Nucleocytoplasmic transport across the nuclear envelope is controlled and facilitated by nuclear pore complexes (NPCs), very large, modular protein assemblies. The Nic96 complex organizes four architectural proteins, Nic96, Nup157/170, Nup188, and Nup192, as well as the more disordered protein Nup53/59. Nup188 is a stacked helical protein with intrinsic flexibility. Moreover, we can show that both Nup188 and Nup192 specifically bind to FG-repeats and translocate across NPCs by facilitated diffusion.

The C-terminal fragment (Nup188C) includes residues 1445–1827, and we solved its structure to 3.0 Å resolution. Nup188C crystallized in space group P212121 with two copies per asymmetric unit. The C-terminal fragment of Nup188, Nup188C, is a right-handed arc-shaped superhelical structure built from 19 helices that form 6 helical repeats, which are stacked in regular order. The first helical pair (α1 and α2) forms a HEAT repeat followed by 5 ARM repeats. The inner face of the structure is built from helices α2, α5, α8, α12, α15, and α19. The C-terminal helix α19 caps the structure. At the N terminus, helices α1 and α2 expose a hydrophobic surface, which strongly suggests that the full-length protein continues in a stacked pattern. This hydrophobic surface engages in a twofold symmetric crystal packing contact with a neighboring Nup188C molecule resulting in a horseshoe-shaped dimer. Because this contact is generated by a protein truncation, we suggest that it is a crystal artifact and not physiologically relevant. Interestingly, the two Nup188C copies in the asymmetrical unit have a different curvature, likely reflecting the intrinsic flexibility of the molecule.

>SLLPKDISQLLSLVSATINGVDNPWSKDQISYFRTLLKVLFVVLRGTKHSNNAAPQKPTAESPVAVTQLVLTTLDRVVARSFRNLAALVHEPDAATTPEDLALITAILQACLSVPGIEQCQLQVLNIMSSHNVLQVATSLFSWSDRLAEKGDPIYGELALLLLLELSALPALAEQLACDGLLGHLTSANLAGFMRRANVSPFTDNAGAARCYAIWAKGILPLLLNILGALGATIAPEVAFVLNQFPNLLRSSVDRLEAPGLSRTVPLSSRDAPGAGPHYFVALVALSEVHSLALLTRVLAALRSGNARDIPEVVWDSGAVLENVEFWLASRKVLRERLLPLNPREAEWRGMKASEGSGCETKLEEKAVGLLEGIRDVLAEEEE[2x]>[16x]GSQIHVDTMKVINDPIHGHIELHPLLVRIIDTPQFQRLRYIKQLGGGYYVFPGASHNRFEHSLGVGYLAGCLVHALGEKQPEL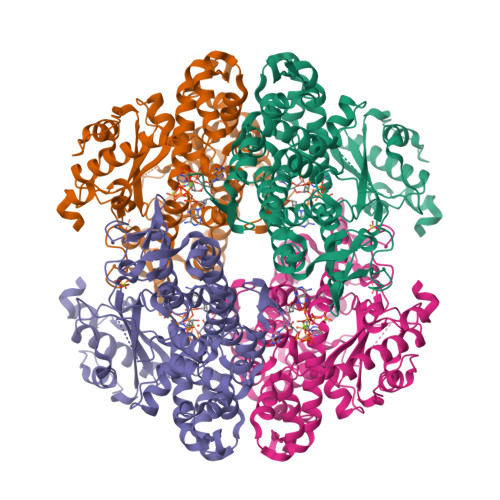QISERDVLCVQIAGLCHDLGHGPFSHMFDGRFIPLARPEVKWTHEQGSVMMFEHLINSNGIKPVMEQYGLIPEEDICFIKEQIVGPLESPVEDSLWPYKGRPENKSFLYEIVSNKRNGIDVDKWDYFARDCHHLGIQNNFDYKRFIKFARVCEVDNELRICARDKEVGNLYDMFHTRNSLHRRAYQHKVGNIIDTMITDAFLKADDYIEITGAGGKKYRISTAIDDMEAYTKLTDNIFLEILYSTDPKLKDAREILKQIEYRNLFKYVGETQPTGQIKIKREDYESLPKEVASAKPKVLLDVKLKAEDFIVDVINMDYGMQEKNPIDHVSFYCKTAPNRAIRITKNQVSQLLPEKFAEQLIRVYCKKVDRKSLYAARQYFVQWCADRNFTKPQDGDVIAPLITPQKKEWNDSTSVQNPTRLREASKSRVQLFKDDPM>GRKERERLEEKLEDANERIAELVKLEERQRIARDLHDTLGQKLSLIGLKSDLARKLIYKDPEQAARELKSVQQTARTSLNEVRKIVSSMKGIRLKDELINIKQILEAADIMFIYEEEKWPENISLLNENILSMCLKEAVTNVVKHSQAKTCRVDIQQLWKEVVITVSDDGTFKGEENSFSKGHGLLGMRERLEFANGSLHIDTENGTKLTMAIPNNSK[2x]

The simplest TCSs comprise a sensory histidine kinase (HK) and a response regulator (RR) component. To address this question we have used the TCS DesK-DesR from B. subtilis as a model. We had previously shown that the HK DesK, a member of the HisKA_3 family, undergoes important conformational changes to switch between phosphatase- and phosphotransfer-competent states. We now report the crystal structures of the DesKC:DesR complex, trapped in the phosphatase and the phosphotransferase functional states.

HK activation leads to autophosphorylation and subsequent switching to its phosphotransferase state. Upon auto-phosphorylation DesKC adopts a strongly asymmetric conformation able to transfer the phosphoryl group to DesR, its downstream RR partner. Comparing the conformation of the phosphorylatable histidine between HKs performing auto-phosphorylation, and the phosphotransferase complex (this study), the His residue shows ~180° flipping of its imidazole side chain. During auto-phosphorylation, HisNδ1 has been observed to H-bond with the ultra-conserved acidic His + 1 residue, which corresponds to Asp189(HK) in DesK. Once phosphorylated, the His disrupts its contact with this neighbor carboxylate group, stabilizing the P~HK species and leading to His χ−2 dihedral angle flipping. Subsequent re-protonation of His188Nδ1, triggered by RR binding, is consistent with P-N bond weakening, as a first step towards phosphotransfer.>KAPPLVNLAEEKDVKVTVGENMDLKNADLLTDGDKYYLQHDATGNKEGNNWENYQEQGTEVTSTAEGKNGVWVQVDLGASYPLEVINLKRQVYDGQATIGNGNPSGQGKRLKGTKISYKNTAIVIGNEEDLSDGQIVYYEGNPTLPDGVKQPENVSKPYEEAMGGQWFYMDYANKNGLGATELGTTKEARYIRVYTENPKGAAVKFMELGIYGYENEQDVQSQDGPRRVIDNEHPMMIATAYSNDVYEIGQEEGPELQGSNTVDGRWNAIPDDLKENNVLLLHTNNLRQFAPDHIGQAYLQAFHEHGLQIAYEQGAPIMLLGLTAAATPENGGTQYNITADMDYGWLDLMYRMYPNMQGVFNTENFWAGIHPPCEGSAKMLEIADRFGGFFVWSDQDHGSTVTNIVSNANMKKALEKHGDAFYLIYKNTSSNQPDDLKTSSFFQGSWLAGYTGGWGMLSDTWAWDKQFSKLWQGAGSYNNWQRLCGEPEALLGMQMMSTYLGGGVIYTFEFPEIVYGTSNTNSPANTHVLTELFRYIVNHPAPSKKEIMEETKAVLYGNVSSDFYSGLSGKPTGFQIYETGRYGIIPVIPTWGTRAEVTKKLIQEADKLGVTPPNVLDVKDKNLSGQAKQKYFKDLYPIEYVGNAFADKWEGTWYLYNNKVNTNEKQHAILPLEGEEESARLKVEMEPHEFMIMNESGDGTAMDITLNNYRVNKDEIIFDNKFGLTWTGDFSPGQTTINGKLSVYKYMDEYNVVNAPEGKL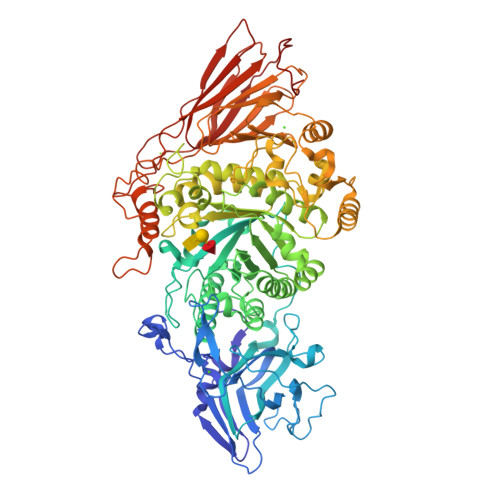SPEDNELRTTTFELTKLAKEPKVQVVKGQQPDTDGQPQYTEPKVEFNEETGKAVITIQTNGWVDLSITGLEFVYDENAQKIEDEP[2x]> GSHGTT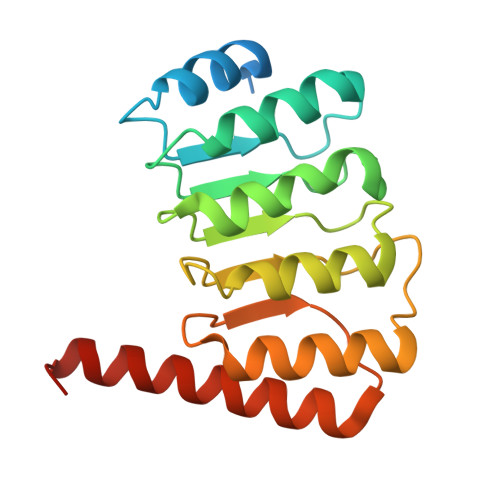FNGIMQSYVPRIVPDEPDNDTDVESCINRLREDDTDLKEVNINNMKRVSKERIRSLIEAACNSKHIEKFSLANTAISDSEARGLIELIETSPSLRVLNVESNFLTPELLARLLRSTLVTQSIVEFKADNQRQSVLGNQVEMDMMMAIEENESLLRVGISFASMEARHRVSEALERNYERVRLRRLGKDPNV> MVEATAQETDRPRFSFSIAAREGKARTGTIEMKRGVIRTPAFMPVGTAATVKALKPETVRATGADIILGNTYHLMLRPGAERIAKLGGLHSFMGWDRPILTDSGGFQVMSLSSLTKQSEEGVTFKSHLDGSRHMLSPERSIEIQHLLGSDIVMAFDEVTPYPATPSRAASSMERSMRWAKRSRDAFDSRKEQAENAALFG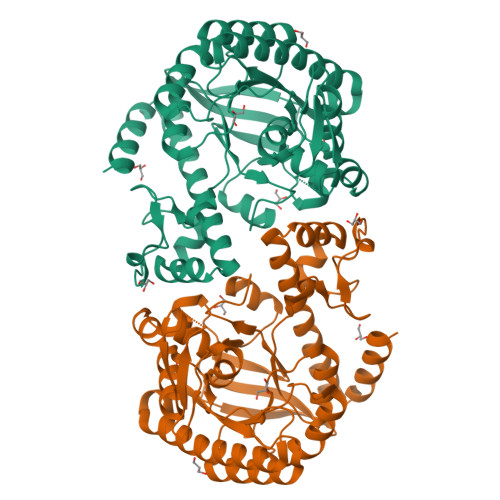IQQGSVFENLRQQSADALAEIGFDGYAVGGLAGGEGQDEMFRVLDFSVPMLPDDKPHYLMGVGKPDDIVGAVERGIDMFDCVLPTRSGRNGQAFTWDGPINIRNARFSEDLKPLDSECHCAVCQKWSRAYIHHLIRAGEILGAMLMTEHNIAFYQQLMQKIRDSISEGRFSQFAQDFRARYFARNS6-[(7-nitro-2,1,3-benzoxadiazol-4-yl)sulfanyl]hexan-1-ol 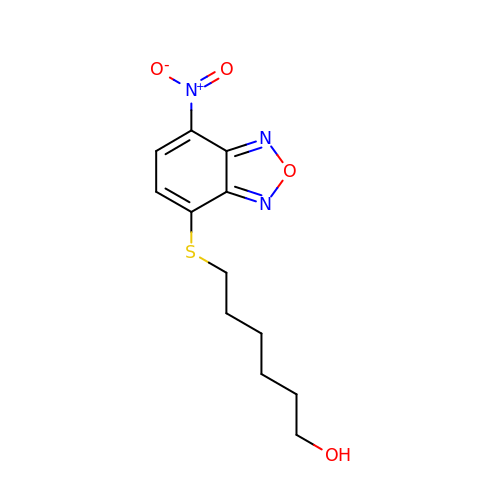| C12 H15 N3 O4 S | RGXYYAZGELLKDA-UHFFFAOYSA-N>DNSYKMDYPEMGLCIIINNKNFHKSTGMTSRSGTDVDAANLRETFRNLKYEVRNKNDLTREEIVELMRDVSKEDHSKRSSFVCVLLSHGEEGIIFGTNGPVDLKKITNFFRGDRCRSLTGKPKLFIIQACRGTELDCGIET[2x];>CHKIPVEADFLYAYSTAPGYYSWRNSKDGSWFIQSLCAMLKQYADKLEFMHILTRVNRKVATEFESFSFDATFHAKKQIPCIVSMLTKEL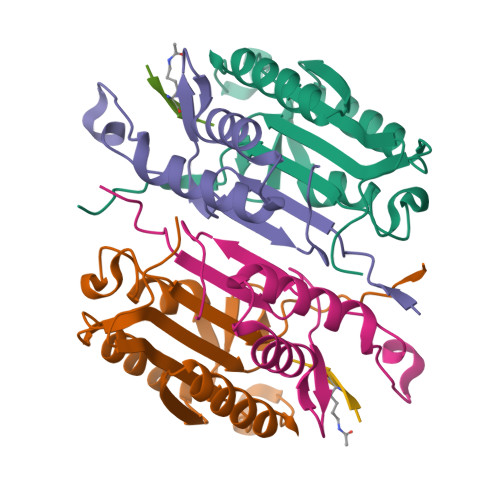YFYHH[2x];>XVDKVD[2x]> MTEEVDFLGQDSDGGSEEVVLTPAELIERLEQAWMNEKFAPELLESKPEIVECVMEQLEHMEENLRRAKREDLKVSIHQMEMERIRYVLSSYLRCRLMKIEKFFPHVLEKEKTRPEGEPSSLSPEELAFAREFMANTESYLKNVALKHMPPNLQKVDLFRAVPKPDLDSYVFLRVRERQENILVEPDTDEQRDYVIDLEKGSQHLI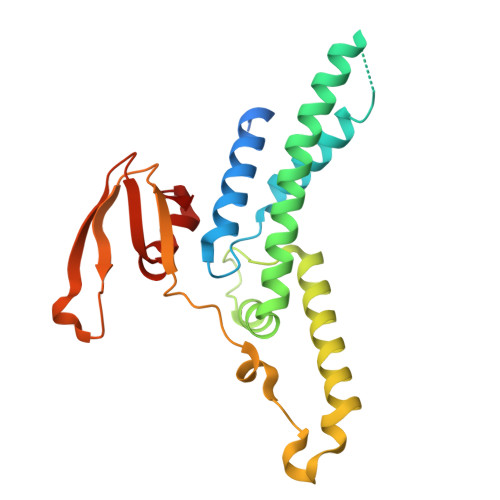RYKTIAPLVASGAVQLI> MNHKVHHHHHHMLDIGNASKTNYGVSLNEYIKLQQRNNPSNYSYSEFEKYINPAKATNKLQFLRIDKFRSVNVSGLSSRLSNKGVLTGQGQAFVNAAKAFNIDPIYLVAQCLHETGNGTSKLAKGVTITEIADESKPIYNGNGQLVGYHMIKLSKPVTVYNLFGIGAKDNSSVFPNRALILGTTYAYNRGWTSIENAIKGAAEFVSLNYVHSSRYSQNTLYKMRYNQNVSNIWHQYATT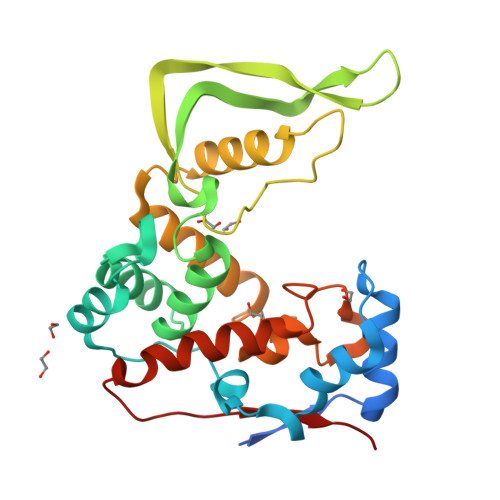PWYASSIADIMRSYQDLYLENNFTFDVPVFAG>[2x]MGAEIPKEMLRAQTNVILLNVLKQGDNYV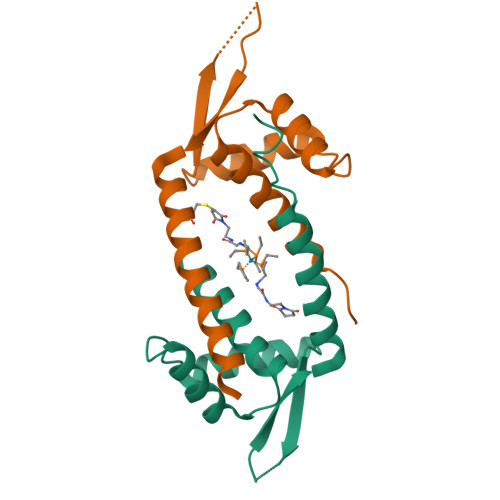YGIIKQVKEASNGEMELNEATLYTIFDRLEQDGIISSYWGDESQGGRRKYYRLTEIGHENCRLAFESWSRVDKIIENLEANKKSEAIK The neural cell adhesion molecule (NCAM) is the prototype and founding member of the immunoglobulin (Ig) superfamily cell adhesion molecules (CAMs). NCAM is present on the cell surface of neurons, astrocytes and oligodendrocytes, where it mediates homophilic and heterophilic cell adhesion. NCAM is involved in neuronal migration, axon growth and guidance, as well as in synaptic plasticity associated with learning and memory. We conclude that the NCAM–FGFR1 interaction at the cell surface may be transient or stabilised by avidity effects resulting from receptor clustering and that conformational changes within NCAM may have a profound role in FGFR1 activation.

When examined by size-exclusion chromatography, all three mutants eluted as a mixture of monomers and dimers, similar to the wild-type protein (data not shown). We obtained crystals of the M610R mutant and determined its structure at 2.7-Å resolution by molecular replacement. The relative orientation of the two FN3 domains in the M610R mutant is less severely bent than in the wild-type structure but still far from fully extended (interdomain angle ∼ 120°). There is no domain interface to speak of in the mutant (240 Å2 buried), and the conformation appears to be stabilised entirely by the crystal lattice. The conformation of multidomain proteins often is influenced by the crystal lattice. The neuroglian tandem, which has an extensive domain interface that incorporates a bound sodium ion, adopts a conformation that is intermediate between the two conformations we report for the NCAM tandem.

>APLAQADTPSSPSIDQVEPYSSTAQVQFDEPEATGGVPILKYKAEWRAVGEEVWHSKWYDAKEASMEGIVTIVGLKPETTYAVRLAALNGKGLGEISAASEFKTQPVREPSAPKLEGQRGEDGNSIKVNLIKQDDGGSPIRHYLVRYRALSSEWKPEIRLPSGSDHVMLKSLDWNAEYEVYVVAENQQGKSKAAHFVFRTAAAHHHHHH[6x]~{N}-(4-ethoxyquinazolin-2-yl)propanamide | C13 H15 N3 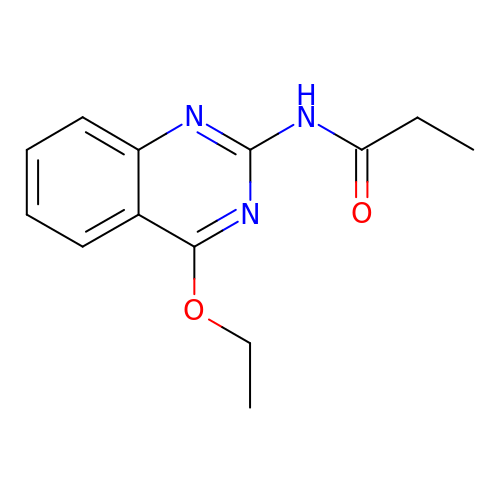O2 | BLXSSFGQMIYBHD-UHFFFAOYSA-N> SNRLDGKVAIITGGTLGI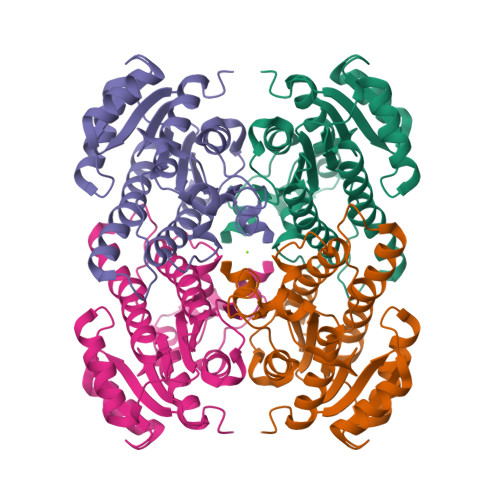GLAIATKFVEEGAKVMITGRHSDVGEKAAKSVGTPDQIQFFQHDSSDEDGWTKLFDATEKAFGPVSTLVNNAGIAVNKSVEETTTAEWRKLLAVNLDGVFFGTRLGIQRMKNKGLGASIINMSSIEGFVGDPSLGAYNASKGAVRIMSKSAALDCALKDYDVRVNTVHPGYIKTPLVDDLPGAEEAMSDRTKTPMGHIGEPNDIAYICVYLASNESKFATGSEFVVDGGYTAQ>[6x]MRGSHHHHHHGSMASSFSMEKVKRILDAQRTEGPATVLAIGTANPPTCFYEADYPDFYFRVTNCEDKPELKEKFKRISERSAVKKRYLHVTEEILKENPNMCSYRAPSLDARHAILVEEV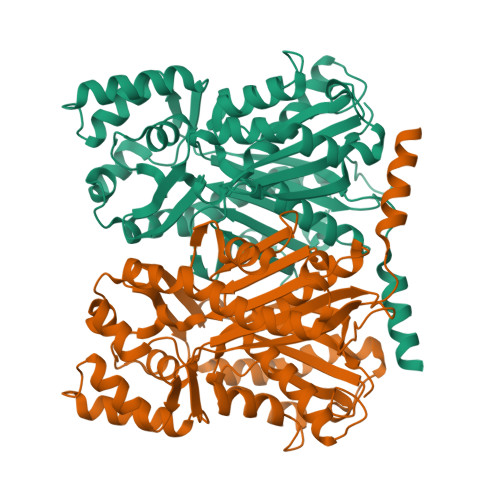PKLGKEAALKAIKEWGQPLSKITHLIFSAMSGVDIPGADFRLMNLLGLEPSVNRLMIYTQGCYMGGAAMRHAKDIAENNAGARVLLVFCDLMDMYFHAPQNRVDLLVGQAVFGDGAAALIVGADPDDDCTERPLFQVVSCAERAVPGTQDYIKAHLKEMGMELHLSTDVPRMIGKNIEKLLADAVSPFGISDWNSLFYIVHPGAVAILDQVEENLGLGEDKLRASRYVLSEYGNMGAASVFFILDEMRNKSAEEGKLTTGEGLEWGVLFSFGPGLTVETVVLLSVPLDSNH> MGHGHHHHHHHHHHSSGHIEGRHMLDNEEDIDVILKKSTILNLDINNDIISDISGFNSSVITYPDAQLVPGINGKAIHLVNNESSEVIVHKAMDIEYNDMFN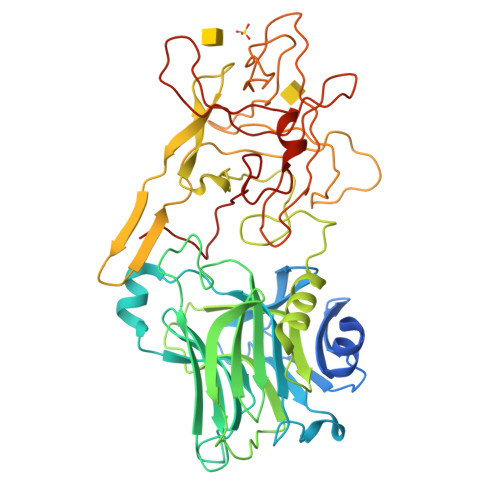NFTVSFWLRVPKVSASHLEQYGTNEYSIISSMKKHSLSIGSGWSVSLKGNNLIWTLKDSAGEVRQITFRDLPDKFNAYLANKWVFITITNDRLSSANLYINGVLMGSAEITGLGAIREDNNITLKLDRCNNNNQYVSIDKFRIFCKALNPKEIEKLYTSYLSITFLRDFWGNPLRYDTEYYLIPVASSSKDVQLKNITDYMYLTNAPSYTNGKLNIYYRRLYNGLKFIIKRYTPNNEIDSFVKSGDFIKLYVSYNNNEHIVGYPKDGNAFNNLDRILRVGYNAPGIPLYKKMEAVKLRDLKTYSVQLKLYDDKNASLGLVGTHNGQIGNDPNRDILIASNWYFNHLKDKILGCDWYFVPTDEGWTND> MKPEVEQELAHILLTELLAYQFASPVRWIETQDVFLKDFNTERVVEIGPSPTLAGMAQRTLKNKYESYDAALSLHREILCYSKDAKEIYYTPDPSELAAKEEPAKEEAPAPTPAASAPAPAAAAPAPVAAAAPAAAAAEIADEPVKASLLLHVLVAHKLKKSLDSIPMSKTIKDLVGGKSTVQNEILGDLGKEFGTTPEKPEETPLEELAETFQDTFSGALGKQSSSLLSRLISSKMPGGFTITVARKYLQTRWGLPSGRQDGVLLVALSNEPAARLGSEADAKAFLDSMAQKYASIVGVDLSSAASASGAAGAGAAAGAAMIDAGALEEITKDHKVLARQQLQVLARYLKMDLDNGERKFLKEKDTVAELQAQLDYLNAELGEFFVNGVATSFSRKKARTFDSSWNWAKQSLLSLYFEIIHGVLKNVDREVVSEAINIMNRSNDALIKFMEYHISNTDETKGENYQLVKTLGEQLIENCKQVLDVDPVYKDVAKPTGPKTAIDKNGNITYSEEPREKVRKLSQYVQEMALGGPITKESQPTIEEDLTRVYKAISAQADKQDISSSTRVEFEKLYSDLMKFLESSKEIDPSQTTQLAGMDVEDALDKDSTKEVASLPNKSTISKTVSSTIPRETIPFLHLRKKTPAGDWKYDRQLSSLFLDGLEKAAFNGVTFKDKYVLITGAGKGSIGAEVLQGLLQGGAKVVVTTSRFSKQVTDYYQSIYAKYGAKGSTLIVVPFNQGSKQDVEALIEFIYDTEKNGGLGWDLDAIIPFAAIPEQGIELEHIDSKSEFAHRIMLTNILRMMGCVKKQKSARGIETRPAQVILPMSPNHGTFGGDGMYSESKLSLETLFNRWHSESWANQLTVCGAIIGWTRGTGLMSANNIIAEGIEKMGVRTFSQKEMAFNLLGLLTPEVVELCQKSPVMADLNGGLQFVPELKEFTAKLRKELVETSEVRKAVSIETALEHKVVNGNSADAAYAQVEIQPRANIQLDFPELKPYKQVKQIAPAELEGLLDLERVIVVTGFAEVGPWGSARTRWEMEAFGEFSLEGCVEMAWIMGFISYHNGNLKGRPYTGWVDSKTKEPVDDKDVKAKYETSILEHSGIRLIEPELFNGYNPEKKEMIQEVIVEEDLEPFEASKETAEQFKHQHGDKVDIFEIPETGEYSVKLLKGATLYIPKALRFDRLVAGQIPTGWNAKTYGISDDIISQVDPITLFVLVSVVEAFIASGITDPYEMYKYVHVSEVGNCSGSGMGGVSALRGMFKDRFKDEPVQNDILQESFINTMSAWVNMLLISSSGPIKTPVGACATSVESVDIGVETILSGKARICIVGGYDDFQEEGSFEFGNMKATSNTLEEFEHGRTPAEMSRPATTTRNGFMEAQGAGIQIIMQADLALKMGVPIYGIVAMAATATDKIGRSVPAPGKGILTTAREHHSSVKYASPNLNMKYRKRQLVTREAQIKDWVENELEALKLEAEEIPSE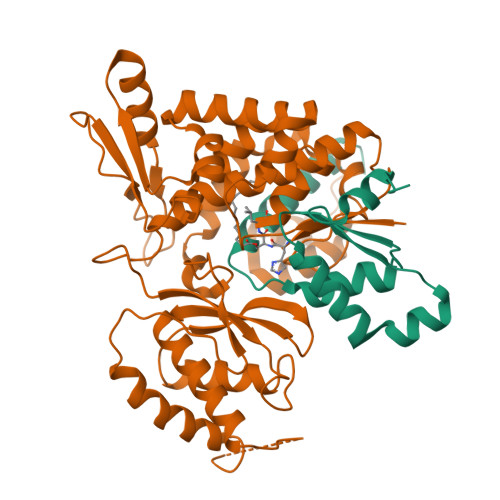DQNEFLLERTREIHNEAESQLRAAQQQWGNDFYKRDPRIAPLRGALATYGLTIDDLGVASFHGTSTKANDKNESATINEMMKHLGRSEGNPVIGVFQKFLTGHPKGAAGAWMMNGALQILNSGIIPGNRNADNVDKILEQFEYVLYPSKTLKTDGVRAVSITSFGFGQKGGQAIVVHPDYLYGAITEDRYNEYVAKVSAREKSAYKFFHNGMIYNKLFVSKEHAPYTDELEEDVYLDPLARVSKDKKSGSLTFNSKNIQSKDSYINANTIETAKMIENMTKEKVSNGGVGVDVELITSINVENDTFIERNFTPQEIEYCSAQPSVQSSFAGTWSAKEAVFKSLGVKSLGGGAALKDIEIVRVNKNAPAVELHGNAKKAAEEAGVTDVKVSISHDDLQAVAVAVSTKK;> MDAYSTRPLTLSHGSLEHVLLVPTASFFIASQLQEQFNKILPEPTEGFAADDEPTTPAELVGKFLGYVSSLVEPSKVGQFDQVLNLCLTEFENCYLEGNDIHALAAKLLQENDTTLVKTKELIKNYITARIMAKRPFDKKSNSALFRAVGEGNAQLVAIFGGQGNTDDYFEELRDLYQTYHVLVGDLIKFSAETLSELIRTTLDAEKVFTQGLNILEWLENPSNTPDKDYLLSIPISCPLIGVIQLAHYVVTAKLLGFTPGELRSYLKGATGHSQGLVTAVAIAETDSWESFFVSVRKAITVLFFIGVRCYEAYPNTSLPPSILEDSLENNEGVPSPMLSISNLTQEQVQDYVNKTNSHLPAGKQVEISLVNGAKNLVVSGPPQSLYGLNLTLRKAKAPSGLDQSRIPFSERKLKFSNRFLPVASPFHSHLLVPASDLINKDLVKNNVSFNAKDIQIPVYDTFDGSDLRVLSGSISERIVDCIIRLPVKWETTTQFKATHILDFGPGGASGLGVLTHRNKDGTGVRVIVAGTLDINPDDDYGFKQEIFDVTSNGLKKNPNWLEEYHPKLIKNKSGKIFVETKFSKLIGRPPLLVPGMTPCTVSPDFVAATTNAGYTIELAGGGYFSAAGMTAAIDSVVSQIEKGSTFGINLIYVNPFMLQWGIPLIKELRSKGYPIQFLTIGAGVPSLEVASEYIETLGLKYLGLKPGSIDAISQVINIAKAHPNFPIALQWTGGRGGGHHSFEDAHTPMLQMYSKIRRHPNIMLIFGSGFGSADDTYPYLTGEWSTKFDYPPMPFDGFLFGSRVMIAKEVKTSPDAKKCIAACTGVPDDKWEQTYKKPTGGIVTVRSEMGEPIHKIATRGVMLWKEFDETIFNLPKNKLVPTLEAKRDYIISRLNADFQKPWFATVNGQARDLATMTYEEVAKRLVELMFIRSTNSWFDVTWRTFTGDFLRRVEERFTKSKTLSLIQSYSLLDKPDEAIEKVFNAYPAAREQFLNAQDIDHFLSMCQNPMQKPVPFVPVLDRRFEIFFKKDSLWQSEHLEAVVDQDVQRTCILHGPVAAQFTKVIDEPIKSIMDGIHDGHIKKLLHQYYGDDESKIPAVEYFGGESPVDVQSQVDSSSVSEDSAVFKATSSTDEESWFKALAGSEINWRHASFLCSFITQDKMFVSNPIRKVFKPSQGMVVEISNGNTSSKTVVTLSEPVQGELKPTVILKLLKENIIQMEMIENRTMDGKPVSLPLLYNFNPDNGFAPISEVMEDRNQRIKEMYWKLWIDEPFNLDFDPRDVIKGKDFEITAKEVYDFTHAVGNNCEDFVSRPDRTMLAPMDFAIVVGWRAIIKAIFPNTVDGDLLKLVHLSNGYKMIPGAKPLQVGDVVSTTAVIESVVNQPTGKIVDVVGTLSRNGKPVMEVTSSFFYRGNYTDFENTFQKTVEPVYQMHIKTSKDIAVLRSKEWFQLDDEDFDLLNKTLTFETETEVTFKNANIFSSVKCFGPIKVELPTKETVEIGIVDYEAGASHGNPVVDFLKRNGSTLEQKVNLENPIPIAVLDSYTPSTNEPYARVSGDLNPIHVSRHFASYANLPGTITHGMFSSASVRALIENWAADSVSSRVRGYTCQFVDMVLPNTALKTSIQHVGMINGRKLIKFETRNEDDVVVLTGEAEIEQPVTTFVFTGQGSQEQGMGMDLYKTSKAAQDVWNRADNHFKDTYGFSILDIVINNPVNLTIHFGGEKGKRIRENYSAMIFETIVDGKLKTEKIFKEINEHSTSYTFRSEKGLLSATQFTQPALTLMEKAAFEDLKSKGLIPADATFAGHXLGEYAALASLADVMSIESLVEVVFYRGMTMQVAVPRDELGRSNYGMIAINPGRVAASFSQEALQYVVERVGKRTGWLVEIVNYNVENQQYVAAGDLRALDTVTNVLNFIKLQKIDIIELQKSLSLEEVEGHLFEIIDEASKKSAVKPRPLKLERGFACIPLVGISVPFHSTYLMNGVKPFKSFLKKNIIKENVKVARLAGKYIPNLTAKPFQVTKEYFQDVYDLTGSEPIKEIIDNWEKYEQS PENTAN-1-OL | C5 H12 O 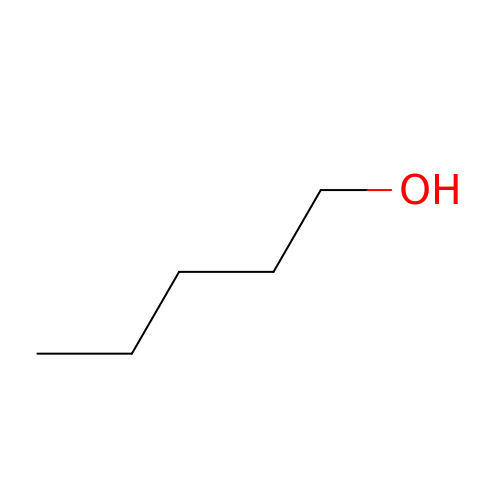| AMQJEAYHLZJPGS-UHFFFAOYSA-N>[2x]MTYTVDESTRPALERFQRFDVDTQLALLWYGYLDLKPQLNPAPPNSVDTPARAVFDHIQDLSQQEQLQAQRDLIKGGSGEINRGYNALSPNAKLEVWL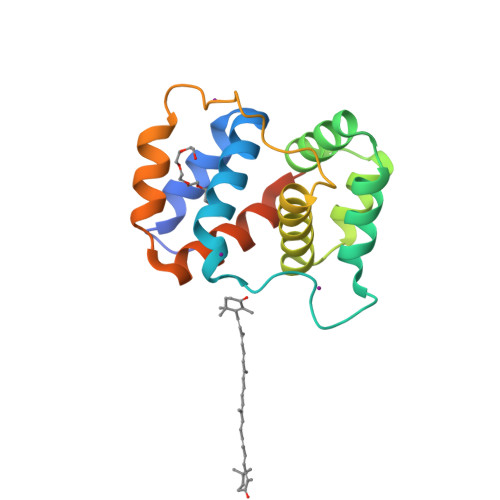LLAQGMENGTIIPMPSDYQLPNGTEEFTAQVKKLEFDQRLNFMLTAVQAMGGSSAHHHHHHHHHH> MAPERLRSR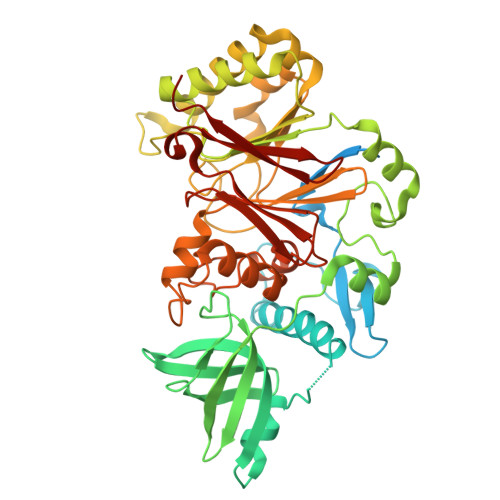ALSAFKLRGLLLRGEAIKYLTEALQSISELELEDKLEKIINAVEKQPLSSNMIERSVVEAAVQECSQSVDETIEHVFNIIGAFDIPRFVYNSERKKFLPLLMTNHPAPNLFGTPRDKAEMFRERYTILHQRTHRHELFTPPVIGSHPDESGSKFQLKTIETLLGSTTKIGDAIVLGMITQLKEGKFFLEDPTGTVQLDLSKAQFHSGLYTEACFVLAEGWFEDQVFHVNAFGFPPTEPSSTTRAYYGNINFFGGPSNTSVKTSAKLKQLEEENKDAMFVFLSDVWLDQVEVLEKLRIMFAGYSPAPPTCFILCGNFSSAPYGKNQVQALKDSLKTLADIICEYPDIHQSSRFVFVPGPEDPGFGSILPRPPLAESITNEFRQRVPFSVFTTNPCRIQYCTQEITVFREDLVNKMCRNCVRFPSSNLAIPNHFVKTILSQGHLTPLPLYVCPVYWAYDYALRVYPVPDLLVIADKYDPFTTTNTECLCINPGSFPRSGFSFKVFYPSNKTVEDSKLQGF>KHSLPDLPYDYGALEPHINAQIMQLHHSKHHAAHVNNLNVTEEKYQEALAKGDVTAQIALQPALKFNGGGHINHSIFWTNLSPNGGGEPKGELLEAIKRDFGSFDKFKEKLTAASVGVQGSGWGWLGFNKERGHLQIAACPNQDPLQGTTGLIPLLGI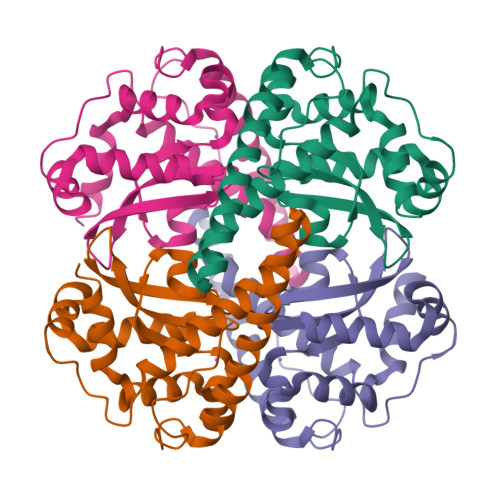DVWEHAYYLQYKNVRPDYLKAIWNVINWENVTERYMACKK[4x]> AVSKGFNYGATKADGSSKYQADFKKDFAAAKALVEGGSGFTSARLYTMIQGGTTNTPIEAIPAAIEEKTELLLGLWASGGNMDNEIAALKSAISQYGDDFANLVVGISVGSEDMYRNSVTGSKSNAGPGVEPEELVSYIQQVRSTIAGTGLSDASIGHVDTWDSWTNSSNSDVVNHLDWLGFDGYPYYQLTMENGIENAKKLFDESVEKTKSVANGKEVWITETGWPVTGPQEGDATASPANAKTYWDEVGCPLFGNTNTWWYMLEDEGASPSFGVVKSDLKT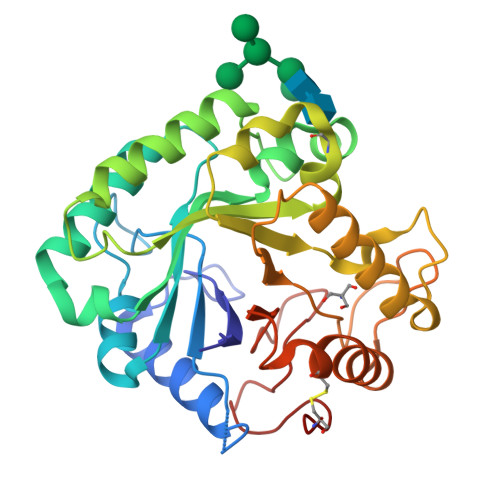PQFDLSC1-(3-chlorophenyl)-2,5-dimethyl-pyrrole-3-carboxylic acid | C13 H12 Cl N 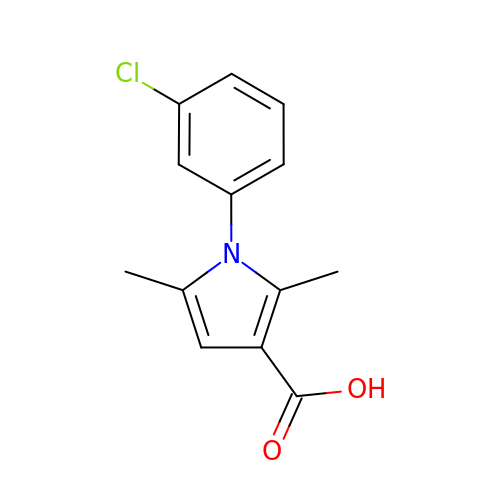O2 | SNPBYQCWMKALIT-UHFFFAOYSA-N> GAMEVEVKLRLLTAAAHLRLTTLLTPYHLKTLHQRNTFFDTPKNDLSLRRAVLRLRFLQNAAVSAASPSPPRCIVSLKAKPTLANGISRVEEDEEEIEYWIGKECVESPAKLSDIGSRVLKRVKEEYGFNDFLGFVCLGGFENVRNVYEWRGVKLEVDETKYDFGNCYEIECETEEPERVKTMIEEFLTEEKIEFSNSDM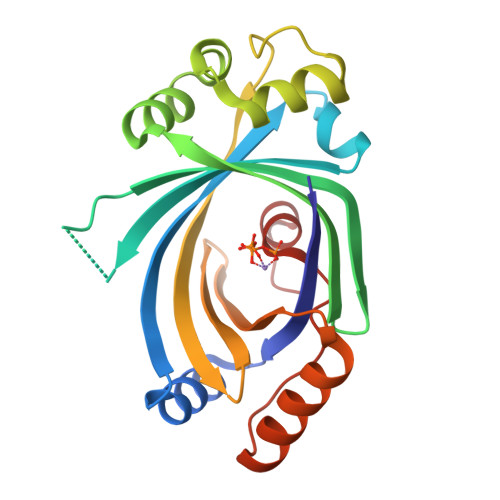TKFAVFRSGKLP>MNRENVR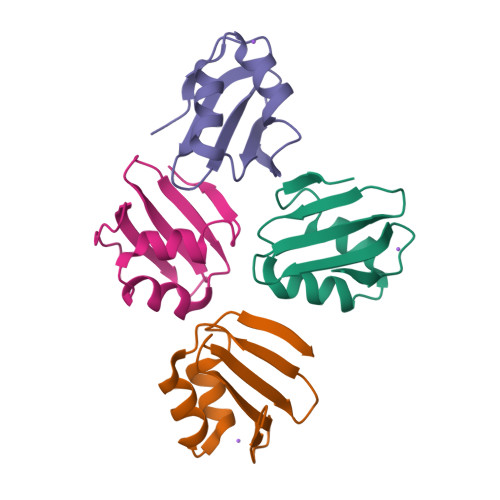SSDLKSVGYDSENKILEVEFNSGGIYQYSTVPEEIYSKLMSSSSHGKYFHKMIRDKYPTKKVK[4x]> MSATKSIVGEALEYVNIGLSHFLALPLAQRISLIIIIPFIYNIVWQLLYSLRKDRPPLVFYWIPWVGSAVVYGMKPYEFFEECQKKYGDIFSFVLLGRVMTVYLGPKGHEFVFNAKLADVSAEAAYAHLTTPVFGKGVIFDCPNSRLMEQKKFVKGALTKEAFKSYVPLIAEEVYKYFRDSKNFRLNERTTGTIDVMVTQPEMTIFTASRSLLGKEMRAKLDTDFAYLYSDLDKGFTPINFVFPNLPLEHYRKRDHAQKAISGTYMSLIKERRKNNDIQDRDLIDSLMKNSTYKDGVKMTDQEIANLLIGVLMGGQHTSAATSAWILLHLAERPDVQQELYEEQMRVLDGGKKELTYDLLQEMPLLNQTIKETLRMHHPLHSLFRKVMKDMHVPNTSYVIPAGYHVLVSPGYTHLRDEYFPNAHQFNIHRWNNDSASSYSVGEEVDYGFGAISKGVSSPYLPFGGGRHRCIGEHFAYCQLGVLMSIFIRTLKWHYPEGKTVPPPDFTSMVTLPTGPAKIIWEKRNPEQKIGGRHHHHHH

A common mechanism of resistance among fungal pathogens occurs due to mutations in the enzymatic target of azole drugs, the cytochrome P450 lanosterol 14α-demethylase (denoted as Erg11p or CYP51). Azoles inhibit the demethylase by coordinating to the heme iron in the active site via a heterocyclic nitrogen atom of an imidazole, triazole or tetrazole ring. In the present study, new high-resolution X-ray crystal structures of the ScErg11p6 × His Y140F mutant in complex with ITC, FLC, VCZ and PCZ and the Y140H mutant in complex with FLC and ITC, along with the wild type ScErg11p6 × His in complex with VCZ, provide evidence that disruption of this hydrogen bond network leads to weaker drug binding. We have created and analysed the structure and function of surrogate triazole resistance phenotypes in the yeast S. cerevisiae by creating Y140F/H single site mutations in lanosterol 14α-demethylase that have homologues in numerous species of pathogenic fungi. This study shows how alterations to a water-mediated hydrogen-bonding network, between the drug and target protein, can affect the affinity of the short-tailed triazole drugs FLC and VCZ but not the long-tailed triazoles ITC and PCZ.

In addition to detecting the mutated residue, a water molecule (843) not present in the wild type structure was found between an oxygen of the ITC 1,3-dioxolane group, the propionates of heme rings A and D and the aromatic side chain of the F140 at distances of 4.0, 3.1, 2.5 and 3.3 Å, respectively. Water 843 replaced the phenolic hydroxyl group of Y140 but, because it makes no polar contacts with the inhibitor, it is unlikely to have any effect on ITC binding. Each mutant crystal structure showed the long tail of the triazole ligand bound within the substrate entry channel in an extended conformation, with the piperazine ring in the chair conformation. This conformation was stabilized via a water-mediated hydrogen bond network between the tetrahedral nitrogen atom N1 of the piperazine ring and the main chain amide nitrogens of H381 and S382. The water mediating this hydrogen bond network resides in a hydrophilic pocket that contains two other waters when ITC or PCZ is bound. The binding of the long-tailed triazoles ITC and PCZ to wild type ScErg11p6 × His and the Y140F/H mutants pushes Y126 to a position so it forms hydrogen bonds with the heme ring D propionate group and the amide nitrogen of F384. The susceptibilities to ITC were comparable for the strains overexpressing the ScErg11p6 × His Y140F, ScErg11p6 × His Y140H or wild type enzyme i.e. 0.09 μg/ml, 0.77 μg/ml and 0.105 μg/ml, respectively. The ScErg11p6 × His Y140F/H mutations disrupt the water-mediated hydrogen bond network between enzyme and both FLC and VCZ. These findings help explain the FLC and VCZ resistance but retention of ITC and PCZ susceptibility in Y140F/H mutants.{[(4-amino-5H-pyrrolo[3,2-d]pyrimidin-7-yl)methyl](hexyl)amino}methanol | C14 H23 N5 O | 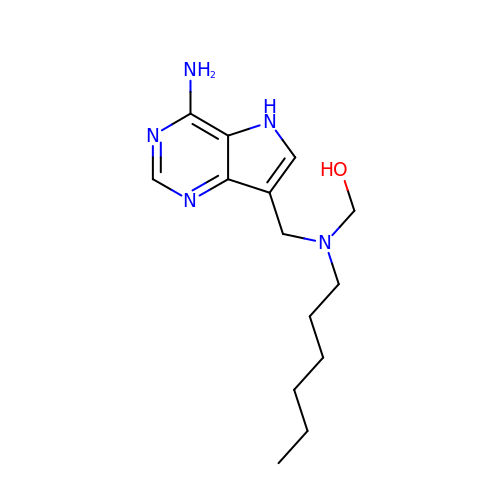OHTIHCJDNXLIDO-UHFFFAOYSA-N>[2x]MKFLTTNFLKCSVKACDTSNDNFPLQYDGSKCQLVQDESIEFNPEFLLNIVDRV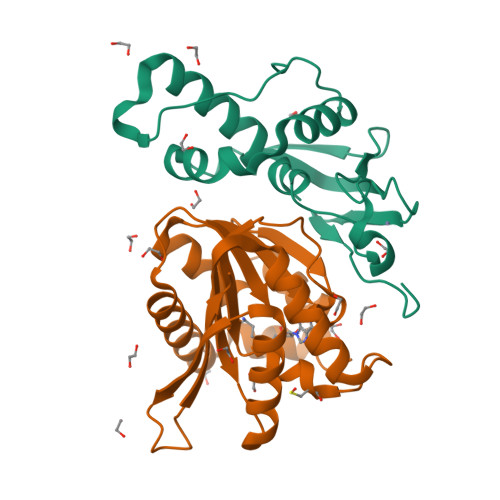DWPAVLTVAAELGNNALPPTKPSFPSSIQELTDDDMAILNDLHTLLLQTSIAEGEMKCRNCGHIYYIKNGIPNLLLPPHLV;>[2x]MSRPEELAPPEIFYNDSEAHKYTGSTRVQHIQAKMTLRALELLNLQPCSFILDIGCGSGLSGEILTQEGDHVWCGLDISPSMLATGLSRELEGDLMLQDMGTGIPFRAGSFDAAISISAIQWLCNADTSYNDPKQRLMRFFNTLYAALKKGGKFVAQFYPKNDDQVDDILQSAKVAGFSGGLVVDDPESKKNKKYYLVLSSGHHHHHH> GSVGPKTGE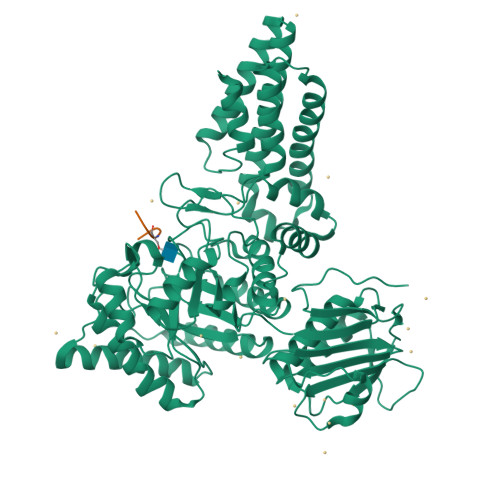ENQVLVPNLNPTPENLEVVGDGFKITSSINLVGEEEADENAVNALREFLTANNIEINSENDPNSTTLIIGEVDDDIPELDEALNGTTAENLKEEGYALVSNDGKIAIEGKDGDGTFYGVQTFKQLVKESNIPEVNITDYPTVSARGIVEGFYGTPWTHQDRLDQIKFYGENKLNTYIYAPKDDPYHREKWREPYPESEMQRMQELINASAENKVDFVFGISPGIDIRFDGDAGEEDFNHLITKAESLYDMGVRSFAIYWDNIQDKSAAKHAQVLNRFNEEFVKAKGDVKPLITVPTEYDTGAMVSNGQPRAYTRIFAETVDPSIEVMWTGPGVVTNEIPLSDAQLISGIYDRNMAVWWNYPVTDYFKGKLALGPMHGLDKGLNQYVDFFTVNPMEHAELSKISIHTAADYSWNMDNYDYDKAWNRAIDMLYGDLAEDMKVFANHSTRMDNKTWAKSGREDAPELRAKMDELWNKLSSKEDASALIEELYGEFARMEEACNNLKANLPEVALEECSRQLDELITLAQGDKASLDMIVAQLNEDTEAYESAKEIAQNKLNTALSSFAVISEKVAQSFIQEALS;> VAHSGAK>[2x]GAMVVKDQVDLRKRKHLEENERRHEDAIKRRKEAVNMNVEKPTVY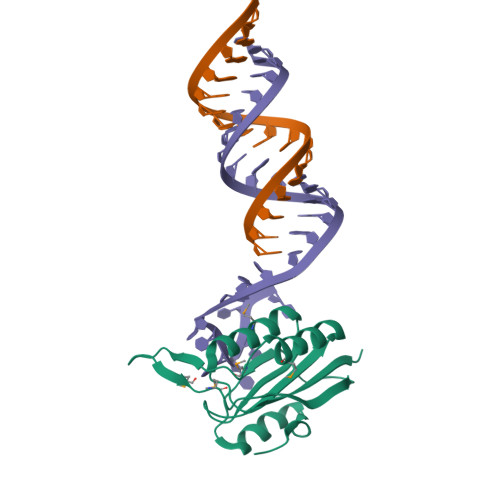HCKVFQFKNLQNPKIRFKLKMNSKELSLKGLCLRIRDDGPGIIIVVGNEKSCKFYENLVMKRIKWNEDFELHTNTGDIKMDMHNNSISKTWEGYLQDCKFKGWFMKVCNDQDSLLRTLGQFDSEHFYSPVQT> 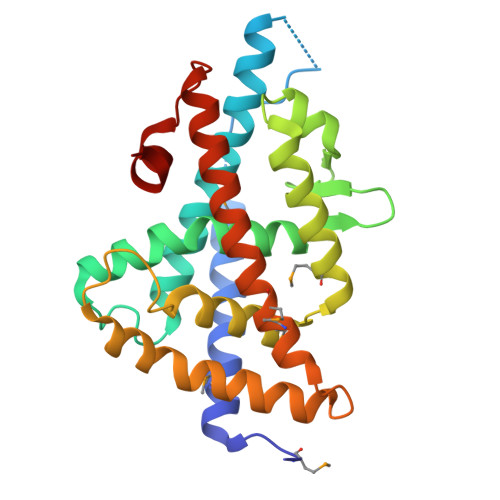GSHMQLTAAQELMIQQLVAAQLQCNKRSFSDQPKVTPWPLGADPQSRDARQQRFAHFTELAIISVQEIVDFAKQVPGFLQLGREDQIALLKASTIEIMLLETARRYNHETECITFLKDFTYSKDDFHRAGLQVEFINPIFEFSRAMRRLGLDDAEYALLIAINIFSADRPNVQEPGRVEALQQPYVEALLSYTRIKRPQDQLRFPRMLMKLVSLRTLSSVHSEQVFALRLQDKKLPPLLSEIWDVHE> LARVAEALGSSEQALRLIVSILMGYPFALFQRYFLFQKETYLIHLYNVFTGLSIAYFNFGMQFFHSLLCVLIQFLILRLMGRTVTAVFTTFVFQMTYLMAGYYFTATEHYDIKWTMPHCVLTLKLIGLAIDYYDGGKDPELLTPEQRRFAVRGVPTLLEVSGFSYFYGAFMVGPQFSMTDYQKLAKGEMTDVPGQRPNSFVPALKRLSLGLLFLVTYTLSSPYISEEYLISDDYMEKPFWFRCGYILVWGKIILYKYVTCWLVTEGVCILVGLGYNGNDQNGKPVWDACANMKVWLYETTPLFTGTIASFNINTNAWVARYVFKRLKFLGNKLLSQALALFFLAIWHGLHSGYLVCFQMELLIVIVERQVINLVRDSPTLSTLASITALQPIFYVLQQTNHWMFM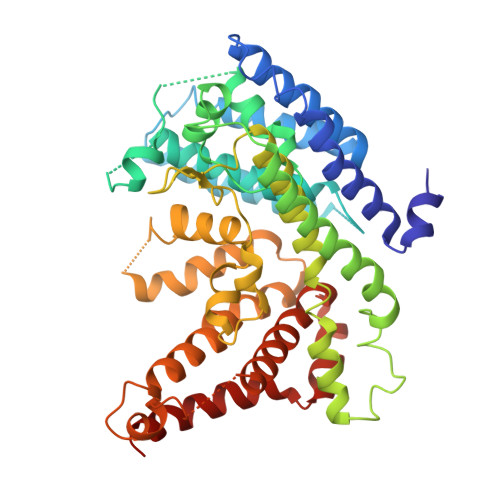GYSLVPFCLFTWDKWMKVYKSIYFLGHVLFFTLLLVLPYIRKL> LQKDSDCCSCQEKWVGYRCNCYFISSEQKTWNESRHLCASQKSSLLQLQNTDELDFMSSSQQFYWIGLSYSEEHTAWLWENGSALSQYLFPSFETFNTKNCIAYNPNGNALDESCEDKNRYICKQ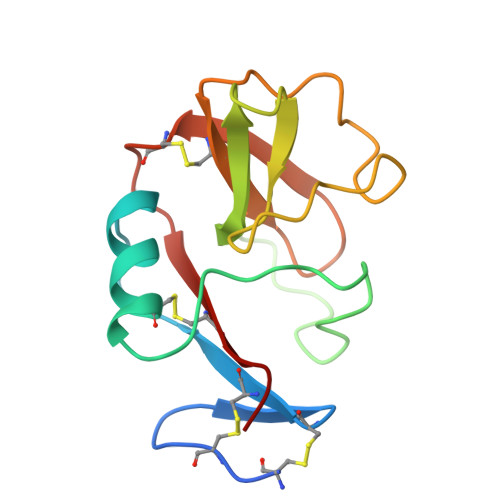QLI> VEDDKEGHLVCRIGDWLQERYEIVGNLGEGTFGKVVECLDHARGKSQVALKIIRNVGKYREAARLEINVLKKIKEKDKENKFLCVLMSDWFNFHGHMCIAFELLGKNTFEFLKENNFQPYPLPHVRHMAYQLCHALRFLHENQLTHTDLKPENILFVNSEFETLYNEHKSCEEKSVKNTSIRVADFGSATFDHEHHTTIVATRHYRPPEVILELGWAQPCDVWSIGCILFEYYRGFTLFQTHENREHLVMMEKILGPIP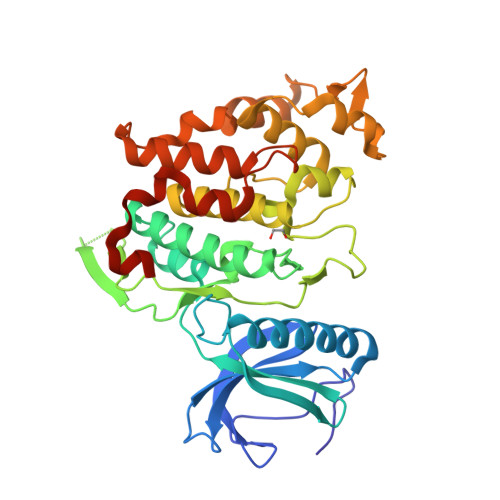SHMIHRTRKQKYFYKGGLVWDENSSDGRYVKENCKPLKSYMLQDSLEHVQLFDLMRRMLEFDPAQRITLAEALLHPFFAGLTPEERSFHTSRNPSR>GRRKPRVLFSQAQVYELER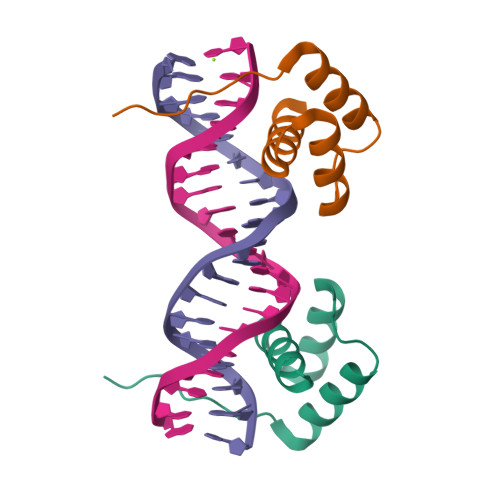RFKQQRYLSAPERDQLASVLKLTSTQVKIWFQNRRYKSK[2x]N-(2-NAPHTHYL)HISTIDINAMIDE | C16 H16 N4 O | 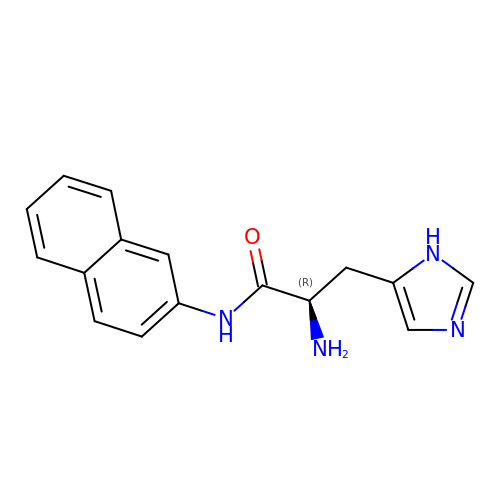DKDILZBBFKZMRO-OAHLLOKOSA-N> MGHHHHHHGNITLTKR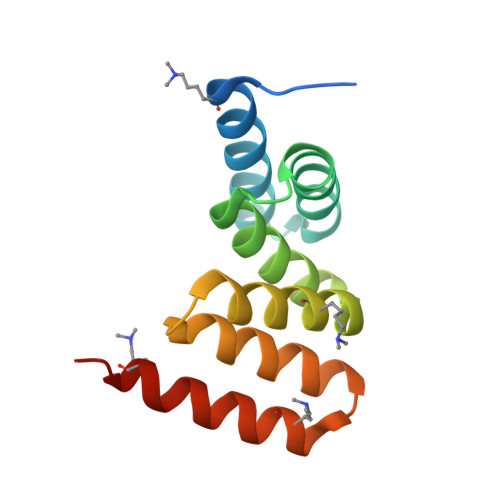QQEFLLLNGWLQLQCGHAERACILLDALLTLNPEHLAGRRCRLVALLNNNQGERAEKEAQWLISHDPLQAGNWLCLSRAQQLNGDLDKARHAYQHYLELKDHNESP> MRYEDRVIFQLEQVATYNPKTSKKENTLITYDAIPCNINPISRARKQLEFGDVKNDVSVLRIKESISYPVSHVLVNGIRYK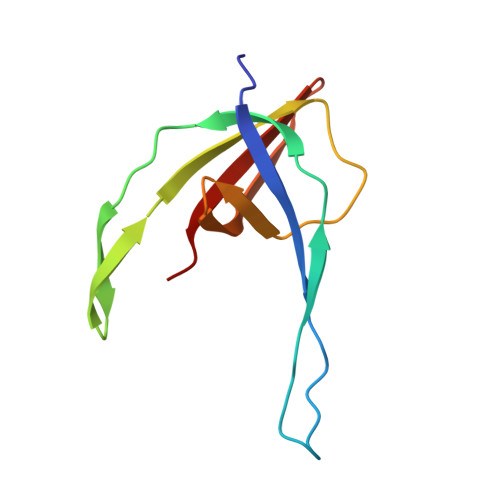IVDTRIYRHETSYYIEEVN>MAMKREQTIENLYQLAQLTQQVQADRIEIVLEERRDEHFPPMSKALMETRSGLTRRKLDEAIAKMEEAGHQFTKNNANHYSISLSEAHMLMDAAGVPKFHERKKNNENKPWIINVQNQKGGTGKSMTAVHLAACLALNLDKRYRICLIDLDPQGSLRLFLNPQISLAEHTNIYSAVDIMLDNVPDGVQVDTEFLRKNVMLPTQYPNLKTISAFPEDAMFNAEAWQYLSQNQSLDIVRLLKEKLIDKIASDFDIIMIDTGPHVDPLVWNAMYASNALLIPCAAKRLDWASTVNFFQHLPTVYEMFPEDWKGLEFVRLMPTMFEDDNKKQVSVLTEMNYLLGDQVMMATIPRSRAFETCADTYSTVFDLTVNDFEGGKKTLATAQDAVQKSALELE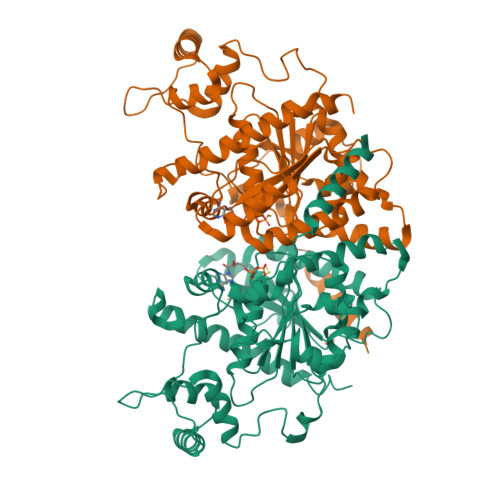RVLHSHWSSLNQG[4x]> MSTSSHTVLLIQTSPRLDSRTWGDYESVTDALDALCKMFEDFLSKKSAAPVTYDVSQVY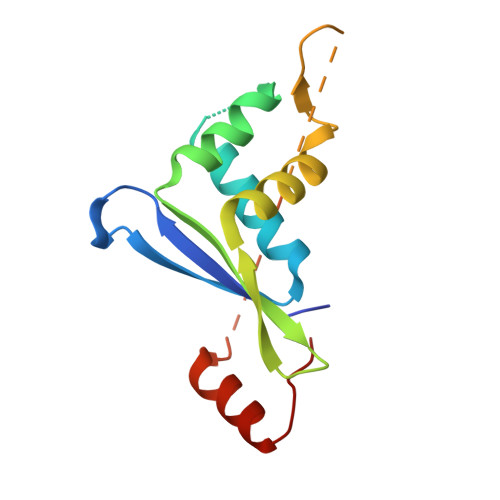EFLDKLSDVSMMIFNRETGQYIGRTRAWIKQQVYEMMRGRCQHPGSSGSSGSSGSSGSSGSSGSSNKRITLNERFGVLEKGYTIQA>[3x]PNWELLSSLGEYKDINLESSNASNITYDLEKYKNLDEGTIVVRFNSKDSKIQSLLGISNSKTKNGYFNFYVTNSRVGFELRNQKNEGNTQ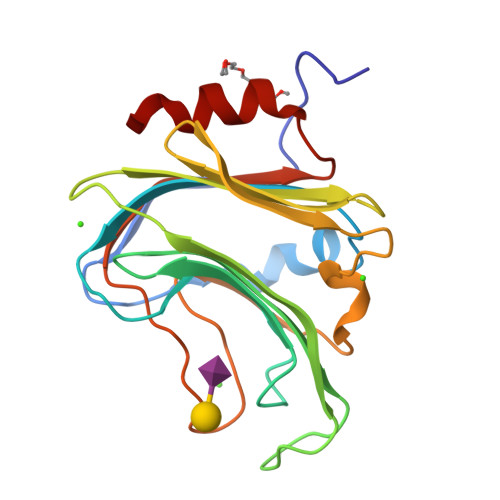NGTENLVHMYKDVALNDGDNTVALKIEKNKGYKLFLNGKMIKEVKDTNTKFLNNIENLDSAFIGKTNRYGQSNEYNFKGNIGFMNIYNEPLGDDYLLSKTGETK>MRINHNIAALNTLNRLPSNNSASQKNMEKLSSGLRINRAGDDAAGLAISEKMRGQIRGLEMASKNSQDGISLIQTAEGALTETHAILQRVRELVVQAGNTGTQDKATDLQSIQDEISALTDEIDGISNRTEFNGKKLLDGTYKVDTATPANQKNLVFQIGANATQQISVNIEDMGADALGIKE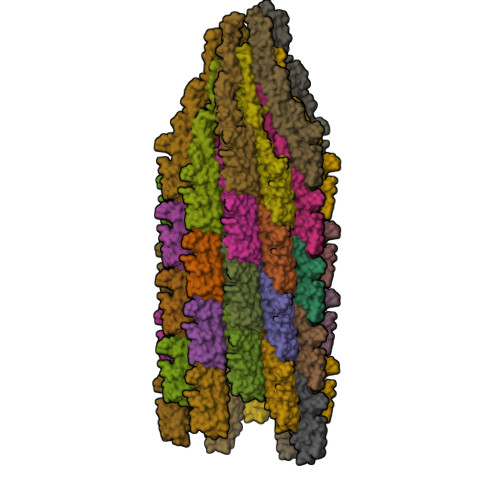ADGSIAALHSVNDLDVTKFADNAADCADIGFDAQLKVVDEAINQVSSQRAKLGAVQNRLEHTINNLSASGENLTAAESRIRDVDMAKEMSEFTKNNILSQASQAMLAQANQQPQNVLQLLR[46x]>QAKHKQRKRLKSSCKRHPLYVDFSDVGWNDWIVAPPGYHAFYCHGECPFPLADHLNSTNHAIVQTLVNSVNSKIPKACCVPTELSAISMLYLDENEKVVLKNYQDMVVEGCGCR[2x];>GSQNLDSMLHGTGMKSDSDQKKSENGVTLAPEDTLPFLKCYCSGHCPDDAINNTCITNGHCFAIIEE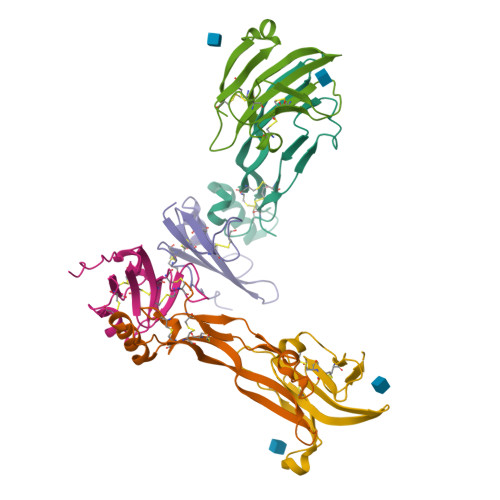DDQGETTLASGCMKYEGSDFQCKDSPKAQLRRTIECCRTNLCNQYLQPTLPPVVIGPFFDGSIR[2x];>AILGRSETQECLFFNANWERDRTNQTGVEPCYGDKDKRRHCFATWKNISGSIEIVKQGCWLDDINCYDRTDCIEKKDSPEVYFCCCEGNMCNEKFSYFPEME[2x]> MAFTRAFLSKSTVEFGQDNFLTC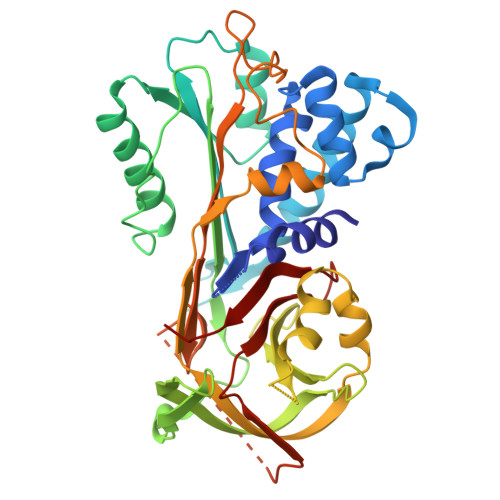PLGILFTLGILLGSGGAQGKTGHQIGKAIRLKSTSSSWNPFGAQEEMKSLYKELNDSLGSEKTFIDDKEEKVVRISTGLFVQRTHEIETSFNESIKNDFKGELIPVNFLNRTSATLSINRWVDQQSNGLLEKFFMDDIPDDTGMILVNVFYFRDFWESPFEPHYTKIENFDISPNRQIKVPMMMKEEVLHYGKFENQGFEIVSKPLNNTRFTFVVVLPLEKWSLTGAMELLNGNKILSEYIKKLKETTVSLRLPKFTLKNTLDLVQTLKSMGIVDLFNPVAANLSGITHDHQLYVDKFMQTNILKLNESGIEATTVTSPIFVPISAVLPDIDFNVNHPFICFIYDQQLTMPIIAAKVIEPIISSA> GPMAWASSFDAFFKNFKRESKIISEYDITLIMTYIEENKLQKAVSVIEKVLRDIESAPLHIAVTGETGAGKSTFINTLRGVGHEEKGAAPTGAIETDMKRTPYPHPKLPNVTIWDLPGIGTTNFTPQNYLTEMKFGEYDFFIIISATRFKENDAQLAKAIAQMGMNFYFVRTKIDSDLDNEQKFKPKSFNKEEVLKNIKDYCSNHLQESLDSEPPVFLVSNVDISKYDFPKLETKLLQDLPAHKRHVFSLSLQSLTEATINYKRDSLKQKVFLEAMKAGALATIPLGGMISDILENLDETFNLYRSYFGLDDASLENIAQDLNMSVDDFKVHLRFPHLFAEHNDESLEDKLFKYIKHISSVTGGPVAAVTYYRMAYYLQNLFLDTAANDAIALLNSKALFEKKVGPYISEPPEYWEA

One prominent IFN-γ inducible event is the upregulation of two subfamilies of IFN-inducible GTPases, immunity-related GTPases (IRGs), and guanylate-binding proteins (GBPs). They specifically target the PV membrane (PVM) and disrupt the PV in which *T. gondii* is enfolded. Upon infection with *Toxoplasma gondii*, host cells produce immune-related GTPases (IRGs) to kill the parasite. *T. gondii* counters this response by releasing ROP18 kinase, which inactivates IRG GTPases and inhibits their recruitment to the *T. gondii* parasitophorous vacuole (PV). The parasite-derived ROP18 phosphorylates host IRGs including Irgb6 at two conserved threonine residues in the switch I region, biochemically abrogating the GTPase activity of IRGs and inhibiting the recruitment of IRGs, thus rendering IRGs inactive.

To assess the effect of phosphorylation of the Thr95 on Irgb6, the amino acid was substituted to aspartate as a phosphomimetic mutation (T95D mutation), following a previous paper. Consequently, Irgb6-WT hydrolyzed two-thirds of GTP to GDP, whereas Irgb6-T95D hydrolyzed only about 10% of GTP to GDP ([Fig fig2]). This indicates that the phospho-mimicking mutation of Thr95 (T95D) in the switch I region of Irgb6 significantly reduced the GTPase activity of Irgb6. The crystal structures of Irgb6-T95D were solved with GTP (Irgb6-T95D-GTP) and without nucleotide (nucleotide free: NF) (Irgb6-T95D-NF) at 1.68 and 2.05 Å resolution, respectively ([Fig fig3] and [Fig fig3] and [Table tbl1]). The former structure possessed GTP in the nucleotide binding pocket ([Fig fig4]). Irgb6-T95D-GTP adopted the same conformation as Irgb6-WT-GTP ([Fig fig3] and [Fig fig3]), with an overall root mean square deviation (RMSD) from Irgb6-WT-GTP of 0.259 Å ([Fig fig3]). As in the Irgb6-WT-GTP structure, Irgb6-T95D-GTP represents a collision complex with GTP in which the switch I and II regions are located away from the γ-phosphate of GTP ([Fig fig4]). Phosphates in GTP are buried in P-loop.> GSGSAMIEARQVSELSTRIISSVQMLSNAQNEQERKEAGRVLFEQLESLLTHIKELGGESFDSKLLDALESNVQNVINNLAELGVTVERKLWLAKEIDTRVEEMRLLSEELEQLTRTQVQNTSTIAVANVTHIYDLLEANKKDQVYQALDALVEVDLDLTERLHELHLLAFKMLNQIEEA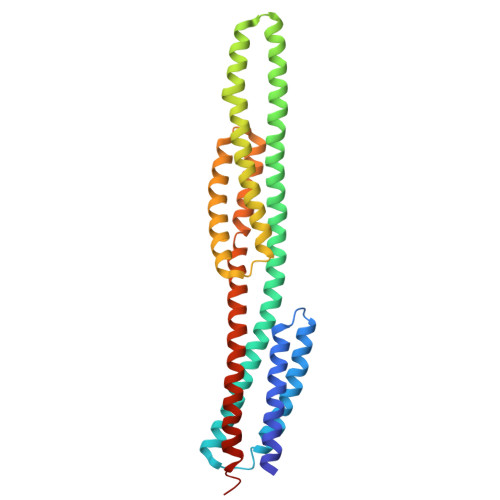RTLTNVDRIQQIQTAFENNLKIMKRRVLAVEDPTRSKQMSQLLTELGKRQVVFTILLQQYENNEQSQQLMQKTLELFSELNSTVNKLVDDSNKTTTK>[2x]HHHHHHSSGLVPRGSHMTKALYDRDGAAIGNLQKLRFFPLAISGGRGARLIEENGRELIDLSGAWGAASLGYGHPAIVAAVSAAAANPAGATILSASNAPAVTLAERLLASFPGEGTHKIWFGHSGSDANEAAYRAIVKATGRSGVIAFAGAYHGCTVGSMAFSGHSVQADAAKADGLILLPYPDPYRPYRNDPTGDAILTLLTEKLAAVPAGSIGAAFIEPIQSDGGLIVPPDGFLRKFADICR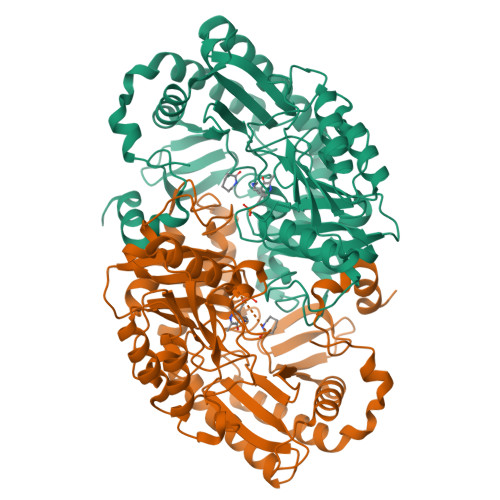AHGILVVCDEVKVGLARSGRLHCFEHEGFVPDILVLGKGLGGGLPLSAVIAPAEILDCASAFAMQTLHGNPISAAAGLAVLETIDRDDLPAMAERKGRLLRDGLSELAKRHPLIGDIRGRGLACGMELVCDRQSREPARAETAKLIYRAYQLGLVVYYVGMNGNVLEFTPPLTITETDIHKALDLLDRAFSELSAVSNEEIAQFAGW3-(2-phenylethyl)-1H-indazole | C15 H14 N2 | 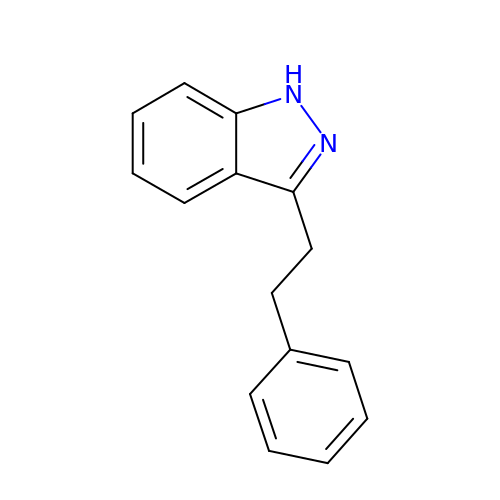LXISBZUPGQAOKP-UHFFFAOYSA-N>[2x]MSVEKIPGYTYGETENRAPFNLEDLKLLKEAVMFTAEDEEYIQKAGEVLEDQVEEILDTAYGFVGSHPHLLYYFTSPDGTPNEKYLAAVRKRFSRWILDTSNRSYDQAWLDYQYEIGLRHHRTKKNQTDNVESVPNIGYRYLVAFIYPITATMKPFLARKGHTPEEVEKMYQAWFKATTLQVALWSYPYVKYGDF

Protoglobin (Pgb) is a recently discovered haem-protein with distinct structural and functional features that make it unique within the globin superfamily. The MaPgb* structure can be considered as an expanded version of the 3/3 helical sandwich typical of “classical” globins (i.e. Mb), with an additional N-terminal extension, built by a 20-residue loop, followed by the Z-helix, which precedes the globin-fold conserved A-helix. Residues belonging to the Z-helix contribute to formation of the Pgb homodimer, which is centered on the intermolecular four-helix bundle built by the G- and H-helices of the two subunits. Thus, in Pgb the access of diatomic ligands, such as O2, CO, and NO, to the haem is granted by two orthogonal apolar tunnels that reach the haem distal region from entry sites at the B/G and B/E helix interfaces.

In the Trp(60)B9Ala mutant one cyanide stabilizing H-bond is absent, while the H-bond to Tyr(61)B10 OH group is maintained (2.82 Å for chain A, and 2.87 Å for chain B). As a result, the cyanide ligand is slightly tilted toward the entrance of tunnel 2, where Tyr(61)B10 is located, with a haem-Fe(III) coordination bond of 2.25 Å and a Fe-C-N angle of 151° for chain A, and 2.27 Å and 122° for chain B. The Trp(60)B9Ala mutation sets tunnel 1 in a constantly open state. Only a minor rearrangement of the Ile(149)G11 side chain occurs within tunnel 1, which is however not sufficient to fill the empty volume left by the Trp→Ala mutation. Interestingly, the location of the Phe(93)E11 side chain in the Trp(60)B9Ala mutant is superimposable to that of the Phe(93)E11 in the MaPgb*(III)-cyanide complex, thus indicating that the presence of the haem-Fe(III)-bound cyanide is enough to induce the Phe(93)E11 side chain rotation; it also suggests that the insertion of Trp(60)B9 side chain into the haem distal site is only a consequence of the cyanide binding to MaPgb*(III) and of the ligand-linked conformational change of Phe(93)E11 side chain. Therefore, ligand binding to the ferric form brings about a ligand-linked conformational change which leads first to a rotation of the Phe(93)E11 side chain; this movement, which is observed for cyanide, azide and imidazole binding (but it is somehow impaired in the case of nicotinamide) creates then the space for a consequent “induced-fit” structural change of Trp(60)B9, which brings the Trp(60)B9 Nε2 atom at H-bonding distance from the haem Fe(III)-bound ligand. Such a sequential mechanism is confirmed by the structure of the ferric cyanide-bound Trp(60)B9Ala mutant, where the ligand is coordinated to the haem-Fe(III) atom and stabilized only by the Tyr(61)B10 OH group, the Phe(93)E11 residue being rotated by about 120° relative to ligand-free MaPgb*(III), even in the absence of Trp(60)B9.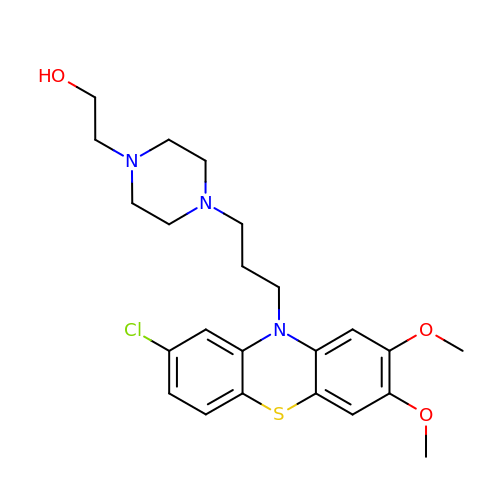2-[4-[3-(8-chloranyl-2,3-dimethoxy-phenothiazin-10-yl)propyl]piperazin-1-yl]ethanol | C23 H30 Cl N3 O3 S | GKWVWOUUPIERSK-UHFFFAOYSA-N> MQNITYSWFVQGMIKATTDAWLKGWDERNGGNLTLRLDDADIAPYHDNFHQQPRYIPLSQPMPLLANTPFIVTGSGKFFRNVQLDPAANLGIVKVDSDGAGYHILWGLTNEAVPTSELPAHFLSHCERIKATNGKDRVIMHCHATNLIALTYVLENDTAVFTRQLWEGSTECLVVFPDGVGILPWMVPGTDAIGQATAQEMQKHSLVLWPFHGVFGSGPTLDETFGLIDTAEKSAQVLVKVYSMGGMKQTISREELI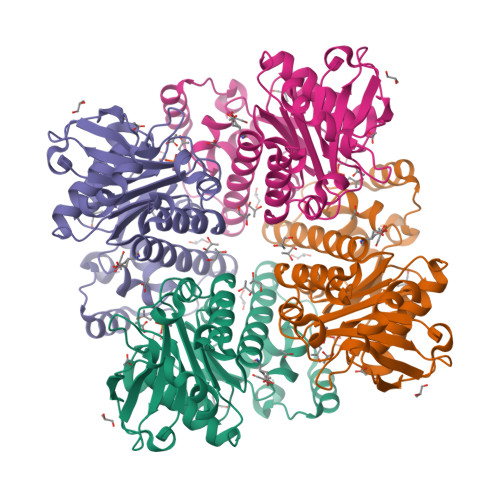ALGKRFGVTPLASALAL> GPGAPNVL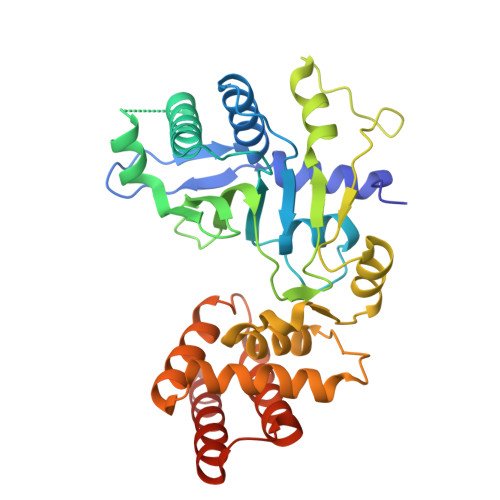NWEQVQRLDGILSETIPIHGRGNFPTLELQPSLIVKVVRRRLAEKRIGVRDVRLNGSAASHVLHQDSGLGYKDLDLIFCADLRGEGEFQTVKDVVLDCLLDFLPEGVNKEKITPLTLKEAYVQKMVKVCNDSDRWSLISLSNNSGKNVELKFVDSLRRQFEFSVDSFQIKLDSLLLFYECSENPMTETFHPTIIGESVYGDFQEAFDHLCNKIIATRNPEEIRGGGLLKYCNLLVRGFRPASDEIKTLQRYMCSRFFIDFSDIGEQQRKLESYLQNHFVGLEDRKYEYLMTLHGVVNESTVCLMGHERRQTLNLITMLAIRVLADQNV>[2x]SLRECELYVQKHNIQALLKDSIVQLCTARPERPMAFLREYFEKLEK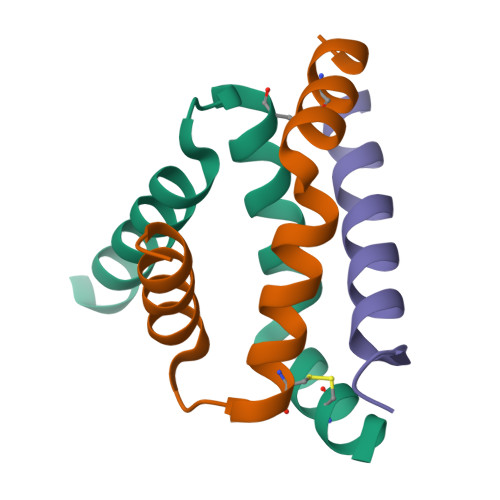EEAK;> TVILEYAHRLSQDILCDALQQWAC(2E)-3-[4-HYDROXY-3-(3-METHOXY-5,5,8,8-TETRAMETHYL-5,6,7,8-TETRAHYDRONAPHTHALEN-2-YL)PHENYL]ACRYLIC ACID | C24 H28 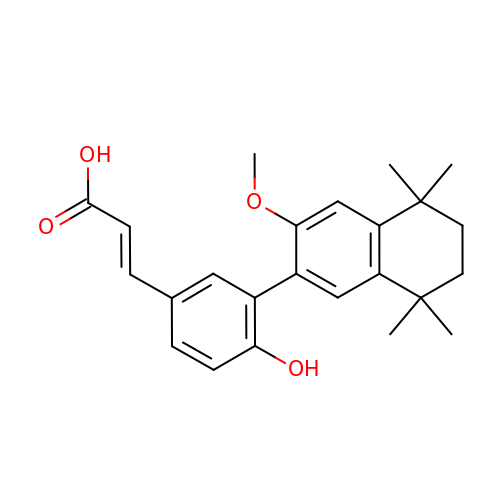O4 | HEFCFLAGDDRJLE-VQHVLOKHSA-N>[2x]GSGNTYYRVVLIGEQGVGKSTLANIFAGVHDSMDSDCEVLGEDT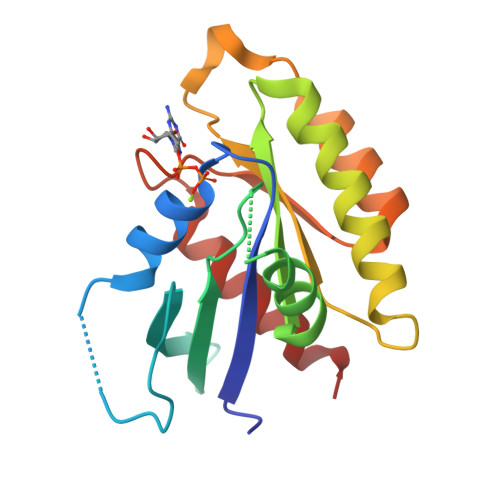YERTLMVDGESATIILLDMWENKGENEWLHDHCMQVGDAYLIVYSITDRASFEKASELRIQLRRARQTEDIPIILVGNKSDLVRCREVSVSEGRACAVVFDCKFIETSAAVQHNVKELFEGIVRQVRLRR> MQICLMDETGATDGALSVLAARWGLEHDEDNPMALVMTPQHLELRKRDEPKLGGIFVDFVGGAMAHRRKFGGGRGEAVAKAVGIKGDYLPDVVDATAGLGRDAFVLASVGCRVRMLERNPVVAALLDDGLTRGYADADIGGWLQERLQLIHASSLTALTDITPRPQVVYLDPMFPHRQKSALVKKEMRVFQSLVGPDLDADGLLEPARQLATK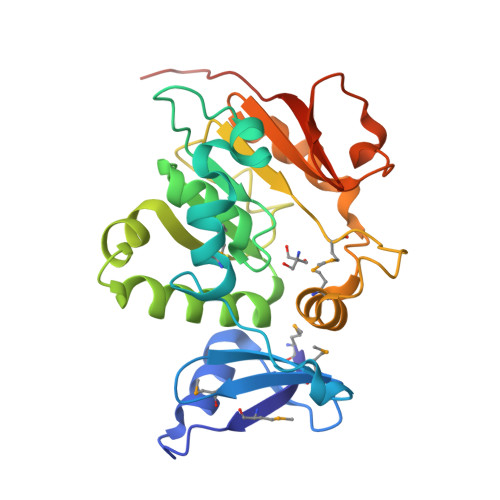RVVVKRPDYAPPLADVATPNAIVTKGHRFDIYAGTPLTELEHHHHHH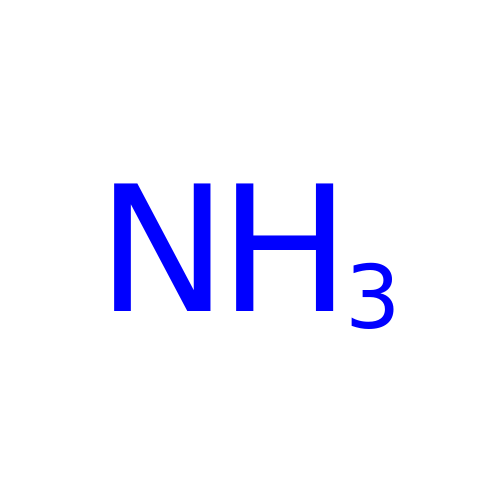AMMONIA | H3 N | QGZKDVFQNNGYKY-UHFFFAOYSA-N> KSPIFGPEEVNSVEGNSVSITCYYPPTSVNRHTRKYWCRQGARGGCITLISSEGYVSSKYAGRANLTNFPENGTFVVNIAQLSQDDSGRYKCGLGINSRGLSFDVSLEVSQGPGLLNDTKVYTVDLGRTVTINCPFKTENAQKRKSLYKQIGLYPVLVIDSSGYVNPNYTGRIRLDIQGTGQLLFSVVINQLRLSDAGQYLCQAGDDSNSNKKNADLQVLKPEPELVYEDLRGSVTFHCALGPEVANVAKFLCRQSSGEN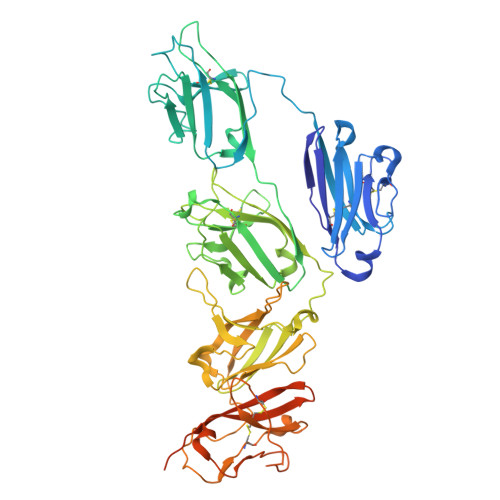CDVVVNTLGKRAPAFEGRILLNPQDKDGSFSVVITGLRKEDAGRYLCGAHSDGQLQEGSPIQAWQLFVNEESTIPRSPTVVKGVAGGSVAVLCPYNRKESKSIKYWCLWEGAQNGRCPLLVDSEGWVKAQYEGRLSLLEEPGNGTFTVILNQLTSRDAGFYWCLTNGDTLWRTTVEIKIIEGEPNLKVPGNVTAVLGETLKVPCHFPCKFSSYEKYWCKWNNTGCQALPSQDEGPSKAFVNCDENSRLVSLTLNLVTRADEGWYWCGVKQGHFYGETAAVYVAVEERKAAGSRDVSLAKADAAPDEKVLDSGFREIENKAIQDPRHHHHHH> AVETDAATTGWATQNGGTTGGAKAAKAVEVKNISDFKKALNGTDSSAKIIKVTGPIDISGGKAYTSFDDQKARSQISIPSNTTIIGVGSNGKFTNGSLVIKGVKNVILRNLYIETPVDVAPHYESGDGWNAEWDAAVIDNSTNVWVDHVTISDGSFTDDKYTTKDGEKYVQHDGALDIKKGSDYVTISYSRFELHDKTILIGHSDSNGSQDSGKLRVTFHNNVFDRVTERAPRVRFGSI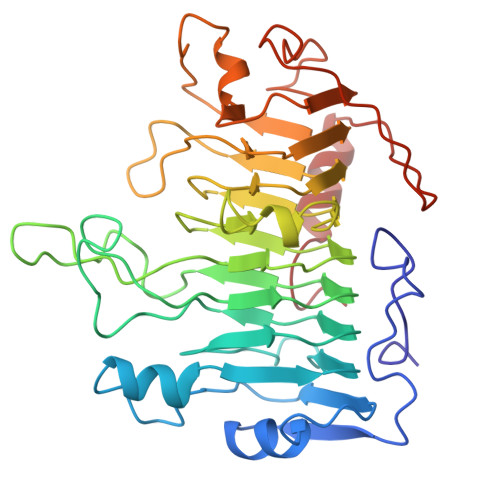HAYNNVYLGDVKHSVYPYLYSFGLGTSGSILSESNSFTLSNLKSIDGKNPECSIVKQFNSKVFSDKGSLVNGSTTTKLDTCGLTAYKPTLPYKYSAQTMTSSLATSINNNAGYGKL> MSSASGLRRGHPAGGEENMTETDAFYKREMFDPAEKYKMDHRRRGIALIFNHERFFWHLTLPERRGTCADRDNLTRRFSDLGFEVKCFNDLKAEELLLKIHEVSTVSHADADCFVCVFLSHGEGNHIYAYDAKIEIQTLTGLFKGDKCHSLVGKPKIFIIQACR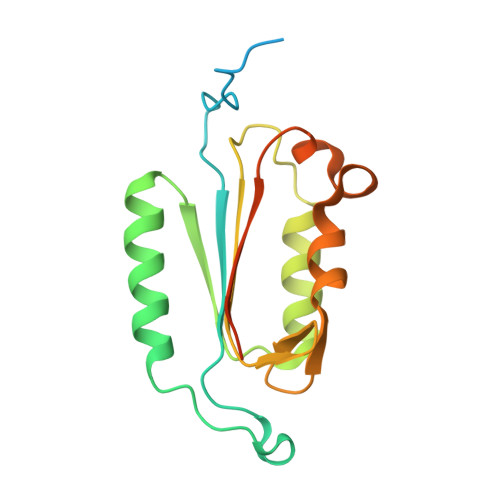GNQHDVPVIPLDVVD> M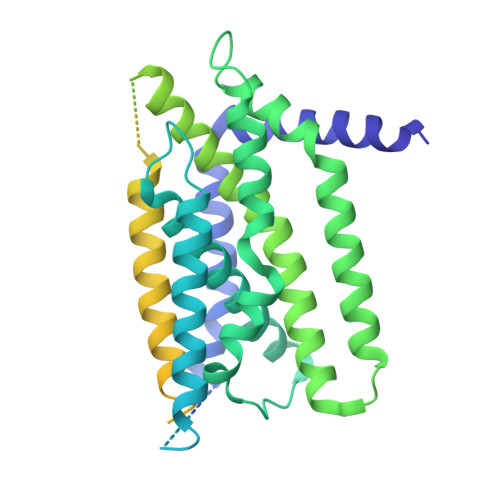TLTERLREKISRAFYNHGLLCASYPIPIILFTGFCILACCYPLLKLPLPGTVPGKYSGVSLYTRKRMVSYTITLVFQHYHAKFLGSLRARLMLLHPSPNCSLRAESLVHVHFKEEIGVAELIPLVTTYIILFAYIYFSTRKIDMVKSKWGLALAAVVTVLSSLLMSVGLCTLFGLTPTLNGGEIFPYLVVVIGLENVLVLTKSVVSTPVDLEVKLRIAQGLSSESWSIMKNMATELGIILIGYFTLVPAIQEFCLFAVVGLVSDFFLQMLFFTTVLSIDIRRMELADLNKRLPPEACLPSAKPVGQPTRYERQLAVRPSTPHTITLQPSSFRNLRLPKRLRVVYFLARTRLAQRLIMAGTVVWIGILVYTDPAGLRNYLAAQVTEQSPLGEGALAPMPVPSGMLPPSHPDPAFSIFPPDAPKLPENQTSPGESPERGGPAEVVHDSPVPEVTWGPEDEELWRKLSFRHWPTLFSYYNITLAKRYISLLPVIPVTLRLNPREALEGRHPQDGRSAWPPPGPIPAGHWEAGPKGPGGVQAHGDVTLYKVAALGLATGIVLVLLLLCLYRVLCP>MKVLFLTANEFEDVELIYPYHRLKEEGHEVYIASFERGTITGKHGYSVKVDLTFDKVNPEEFDALVLPGGRAPERVRLNEKAVSIARKMFSEGKPVASICHGPQILISAGVLRGRKGTSYPGIKDDMINAGVEWVDAEV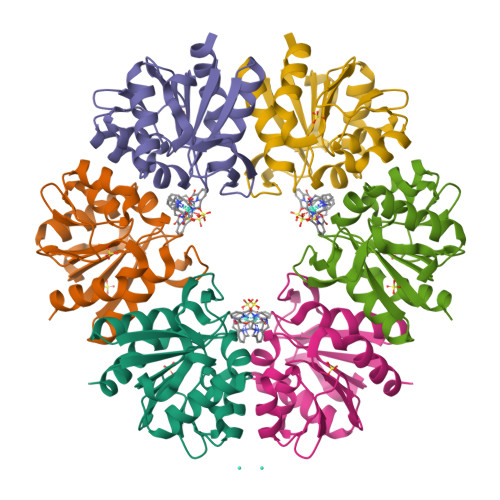VVDGNWVSSRVPADLYAWMREFVKLLK[3x]> VEWTDQERATISSIFGSLDYDDIGPKALSRCLIVYPWTQRHFGSFGNLYNAEAIIGNQKVAAH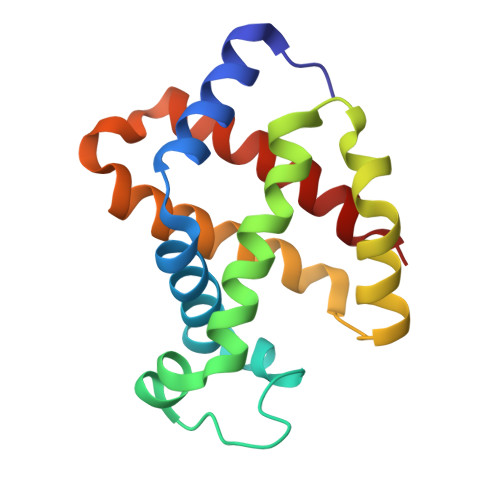GIKVLHGLDRAVKNMDNIKEIYAELSILHSEKLHVDPDNFKLLADCLTIVVAAKMGSGFNPGTQATFQKFLAVVVSALGKQ> SNAMGLFDEVVGAFLKGDAGKYQAILSWVEEQGGIQVLLEKLQSGGLGAILSTWLSNQQRNQSVSGEQLESALGTNAVSDLGQKLGVDTSTASSLLAEQLPKII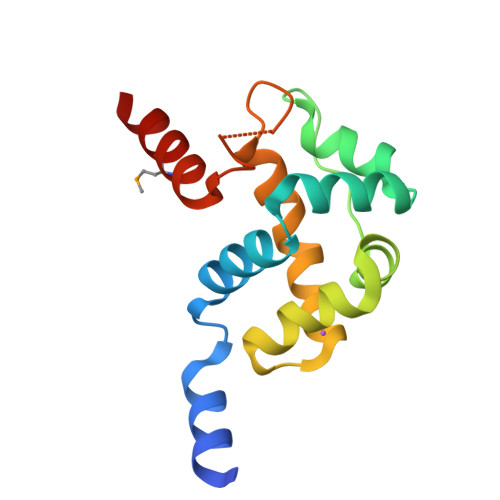DALSPQGEVSAQANNDLLSAGMELLKGKLFR>MPSKLALIQELPDRIQTAVEAAMGMSYQDAPNNVRRDLDNLHACLNKAKLTVSRMVTSLLEKPSVVAYLEGKA[2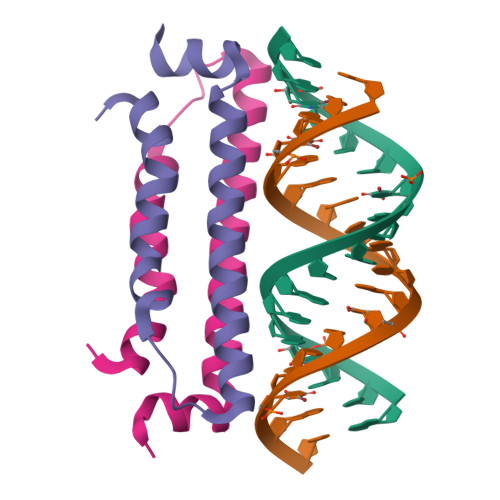x]>[2x]ASNFTQFVLVDNGGTGDVTVAPSNFANGVAEWISSNSRSQAYKVTASVRQSSAQNRKYTIKVEVPKVATHTVGGVELPVAAWRSY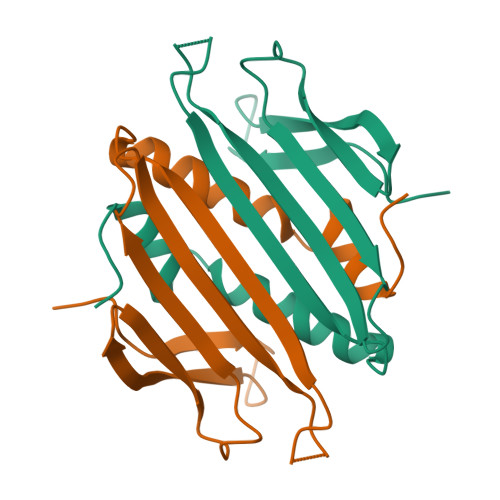LNMELTIPIFATNSDCELIVKAMQGLLKDGNPIPSAIAANSGIY> GNYMGNPWTEYMAKYDIEEVHGSGIRVDLGEDAEVAGTQYRLPSGKCPVFGKGIIIENSNTTFLKPVATGNQDLKDGGFAFPPTNPLISPMTLNGMRDFYKNNEYVKNLDELTLCSRHAGNMNPDNDKNSNYKYPAVYDYNDKKCHILYIAAQENNGPRYCNKDQSKRNSMFCFRPAKDKLFENYTYLSKNVVDNWEEVCPRKNLENAKFGLWVDGNCEDIPHVNEFSANDLFECNKLVFELSASDQPKQYEQHLTDYEKIKEGFKNKNASMIKSAFLPTGAFKADRYKSHGKGYNWGNYNRETQKCEIFNVKPTCLINNSSYIATTA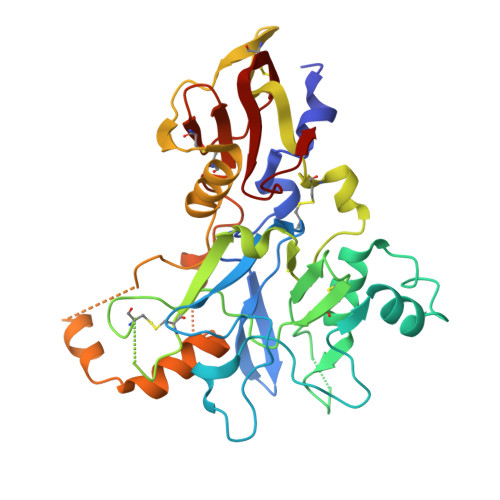LSHPIEVE>[2x]APSYPEYTREEVGRHRSPEERVWVTHG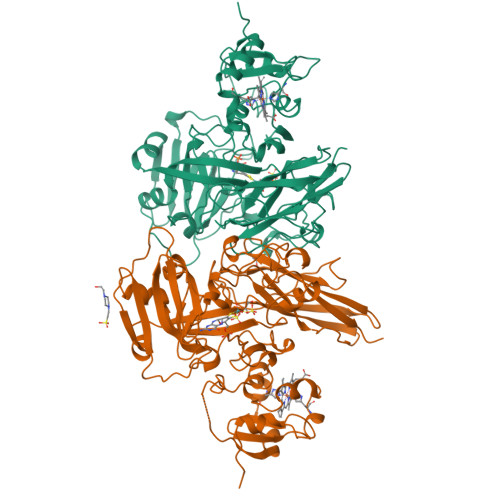TDVFDVTDFVELHPGGPDKILLAAGGALEPFWALYAVHGEPHVLELLQQYKVGELSPDEAPAAPDAQDPFAGDPPRHPGLRVNSQKPFNAEPPAELLAERFLTPNELFFTRNHLPVPAVEPSSYRLRVDGPGGGTLSLSLAELRSRFPKHEVTATLQCAGNRRSEMSRVRPVKGLPWDIGAISTARWGGARLRDVLLHAGFPEELQGEWHVCFEGLDADPGGAPYGASIPYGRALSPAADVLLAYEMNGTELPRDHGFPVRVVVPGVVGARSVKWLRRVAVSPDESPSHWQQNDYKGFSPCVDWDTVDYRTAPAIQELPVQSAVTQPRPGAAVPPGELTVKGYAWSGGGREVVRVDVSLDGGRTWKVARLMGDKAPPGRAWAWALWELTVPVEAGTELEIVCKAVDSSYNVQPDSVAPIWNLRGVLSTAWHRVRVSVQD>MRVVLIVDIVRQEEKLIAKALEENKVQYDIINVAQEPLPFNKALGRYDVAIIRPVSMYRALYSSAVLEAAGVHTINSSDVINVCGDKILTYSKLYREGIPIPDSIIALSAEAALKAYEQRGFPLIDKPPIGSWGRLVSLIRDVFEGKTIIEHRELMGNSALKAHIVQEYIQYKGRDIRCIAIGEELLGCYARNIPPNEWRANVALGGTPSNIEVDEKLKETVVKAVSIVHGEFVSIDILEHPNKGYVVNELNDVPEFKGFMVATNINVAQKLVEYIKENYSK[4x];>[2x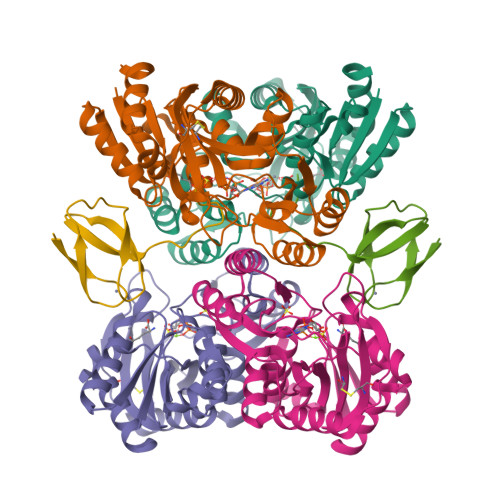]MVVLKCPVCNGDVNVPDDALPGEIVEHECGAQLEVYNDHGRLALRLAEQVGEDWGE>GAMAVAQQLRAESDFEQLPDDVAISANIADIEEKRGFTSHFVFVIEVKTKGGSKYLIYRRYRQFHALQSKLEERFGPDSKSSALACTLPTLPAKVYVGVKQEIAEMRIPALNAYMKSLLSLPVWVLMDEDVRIFFYQSPYDSEQVPQALRRLRPRTRKVKSVSPQGNSVDRMAAPRAEALFDFTGNSKLELNFKAGDVIFLLSRINKDWLEGTVRGATGIFPLSFVKILKDFPEEDDPTNWLRCYYYEDTISTIKDIAVEEDLSSTPLLKDLLELTRREFQREDIALNYRDAEGDLVRLLSDEDVALMVRQARGLPSQKRLFPWKLHITQKDNYRVYNTMP[2x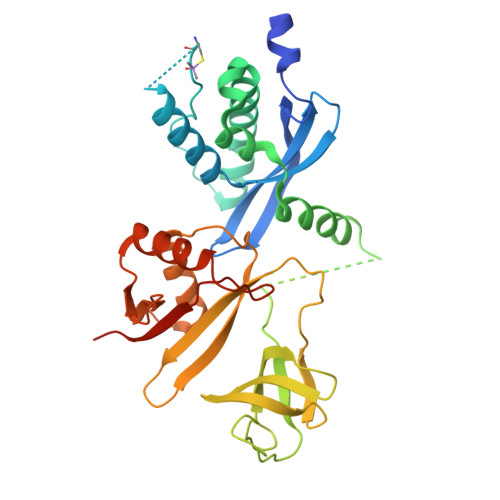]3-methoxybenzyl 3-(piperidin-4-yloxy)-1-benzothiophene-2-carboxylate | C22 H23 N O4 S | 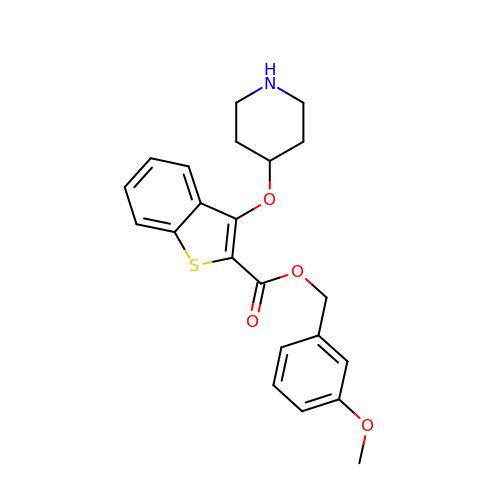GEVWCNOQZDSSIG-UHFFFAOYSA-N>[2x]KPVSLSYRCPCRFFESHVARANVKHLKILNTPNCALQI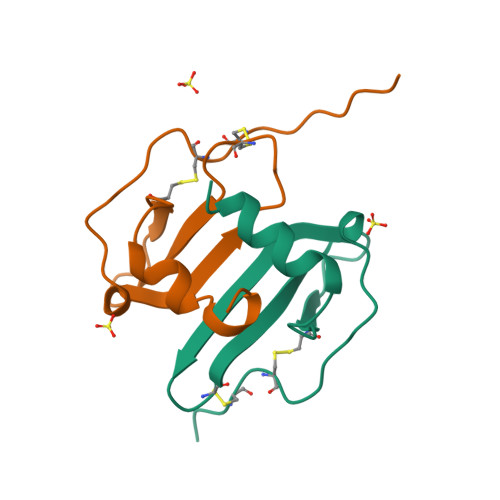VARLKNNNRQVCIDPKLKWIQEYLEKALN> PISPIETVPVKLKPGMDGPKVKQWPLTEEKIKALVEICTEMEKEGKISKIGPENPYNTPVFAIKKKDSTKWRKLVDFRELNKRTQDFWEVQLGIPHPAGLKKNKSVTVLDVGDAYFSVPLDEDFRKYTAFTIPSINNETPGIRYQYNVLPQGWKGSPAIFQSSMTKILEPFKKQNPDIVIYQYMDDLYVGSDLEIGQHRTKIEELRQHLLRWGLTTPDKKHQKEPPFLWMGYELHPDKWTVQPIVLPEKDSWTVNDIQKLVGKLNWASQIYPGIKVRQLCKLLRGTKALTEVIPLTEEAELELAENREILKEPVHGVYYDPSKDLIAEIQKQGQGQWTYQIYQEPFKNLKTGKYARMRGAHTNDVKQLTEAVQKITTESIVIWGKTPKFKLPIQKETWETWWTEYWQATWIPEWE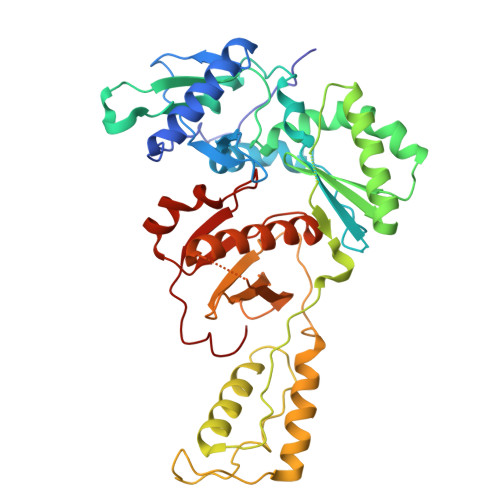FVNTPPLVKLWY> GGYVPAVVIGTGYGAAVSALRLGEAGVQTLMLEMGQLWNQPGPDGNIFCGMLNPDKRSSWFKNRTEAPLGSFLWLDVVNRNIDPYAGVLDRVNYDQMSVYVGRGVGGGSLVNGGMAVEPKRSYFEEILPRVDSSEMYDRYFPRANSMLRVNHIDTKWFEDTEWYKFARVSREQAGK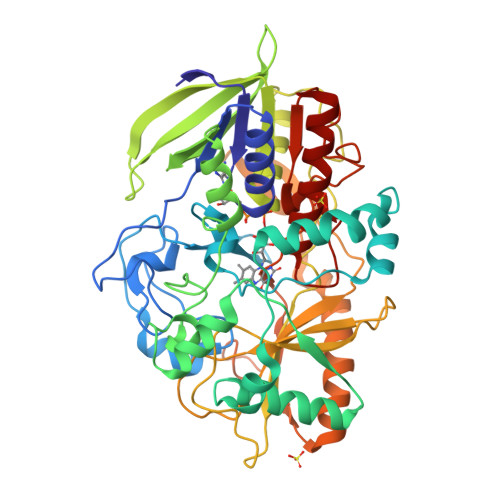AGLGTVFVPNVYDFGYMQREAAGEVPKSALATEVIYGNNHGKQSLDKTYLAAALGTGKVTIQTLHQVKTIRQTKDGGYALTVEQKDTDGKLLATKEISCRYLFLGAGSLGSTELLVRARDTGTLPNLNSEVGAGWGPNGNIMTARANHMWNPTGAHQSSIPALGIDAWDNSDSSVWAEIAPMPAGLETWVSLYLAITKNPQRGTFVYDAATDRAKLNWTRDQNAPAVNAAKALFDRINKANGTIYRYDLFGTQLKAFADDFCYHPLGGCVLGKATDDYGRVAGYKNLYVTDGSLIPGSVGVNPFVTITALAERNVERIIKQDV>[4x]MASMSSSEAPIVQSLEAIPPSQNNQQLAKPEPKWIHLSRYLSKTSQNRVFVDPSGVGHFNSMTWEPPCELLDCGTNYLLKFEVPGIDKKSLSLQYSNNWVIV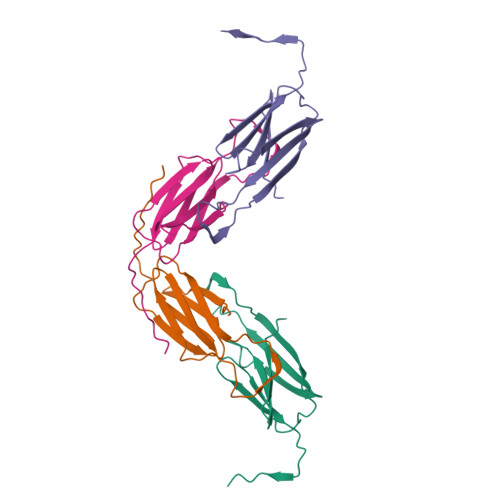SGNKNMPIDEGDFCFTEILYGQFRREVPVPVDASKDGIKAYYQEGILYVKLLKVSNSNWVNVEIV>MGAQVSTQKTGAHETGLNASGNSIIHYTNMNYYKDSASNSANRQEFAQDPGKFTEPVKDIMIKSMPALNSPSAEECGYSDRVRSITLGNSTITTQECANVVVGYGTWPTYLRDEEATAEDQPTQPDVATCRFYTLESVMWQQSSPGWWWKFPDALSNMGLFGQNMQYHYLGRAGYTLHVQCNASKFHQGCLLVVCVPEAEMGCATIANKPDQKSLSNGETANVFDSQNTSGQTAVQANVINAGMGIGVGNLTIFPHQWINLRTNNSATIVMPYVNSVPMDNMFRHNNFTLMIIPFAPLSYSTGATTYVPITVTVAPMCAEYNGLRLAGRQGLPTMLTPGSNQFLTSDDFQSPSAMPQFDVTPEMAIPGQVNNLMEIAEVDSVVPVNNTEGKVMSIEAYQIPVQSNSTNGSQVFGFPLIPGASSVLNRTLLGEILNYYTHWSGSIKLTFMFCGSAMATGKFLLAYSPPGAGAPTTRKEAMLGTHVIWDVGLQSSCVLCIPWISQTHYRYVVMDEYTAGGYITCWYQTNIVVPADTQSDCK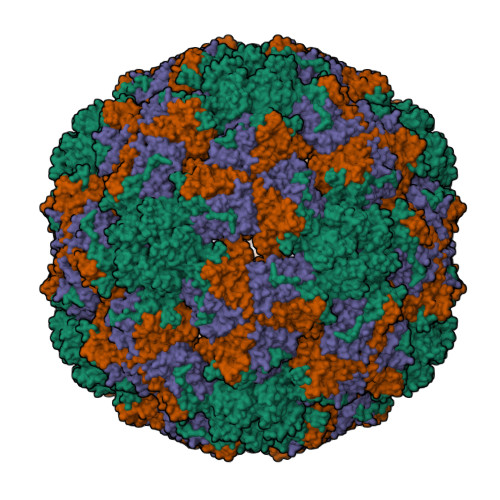ILCFVSACNDFSVRMLKDTPFIKQDSFFQGPPGEAIERAIARVADTISSGPVNSESIPALTAAETGHTSQVVPADTMQTRHVKNYHSRSESTVENFLCRSACVYYTTYKNHGTDGDNFAQWVINTRQVAQLRRKLEMFTYARFDLELTFVITSSQEQSTIKGQDSPVLTHQIMYVPPGGPVPTKINSYSWQTSTNPSVFWTEGSAPPRISIPFISIGNAYSMFYDGWARFDKQGTYGINTLNNMGTLYMRHVNDGSPGPIVSTVRIYFKPKHVKTWVPRPPRLCQYQKAGNVNFEPSGVTEGRTEITAMQTT[3x]>[2x]MAQVINTNSLSLITQNNINKNQSALSSSIERLSSGLRINSAKDDAAGQAIANRFTSNIKGLTQAARNANDGISVAQTTEGALSEINNNLQRIRELTVQASTGTNSDSDLDSIQDEIKSRLDEIDRVSGQTQFNGVNVLAKDGSMKIQVGANDGQTITIDLKKIDSDTLGLNGFNVNGKGETANTAATLKDMSGFTAAAAPGGTVGVTQYTDKSAVASSVDILNAVAGADGNKVTTSADVGFGTPAAAVTYTYNKDTNSYSAASDDISSANLAAFLNPQARDTTKAT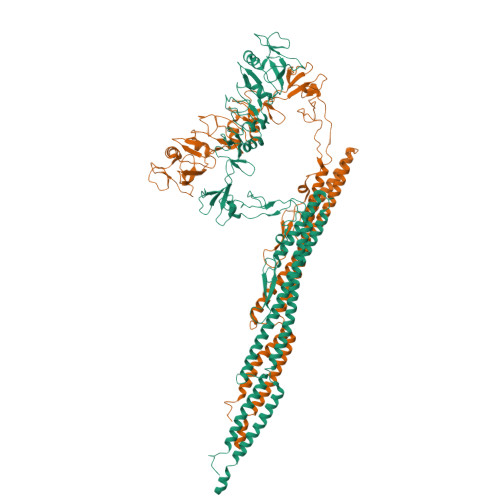VTIGGKDQDVNIDKSGNLTAADDGAVLYMDATGNLTKNNAGGDTQATLAKVATATGAKAATIQTDKGTFTSDGTAFDGASMSIDANTFANAVKNDTYTATVGAKTYSVTTGSAAADTAYMSNGVLSDTPPTYYAQADGSITTTEDAAAGKLVYKGSDGKLTTDTTSKAESTSDPLAALDDAISQIDKFRSSLGAVQNRLDSAVTNLNNTTTNLSEAQSRIQDADYATEVSNMSKAQIIQQAGNSVLAKANQVPQQVLSLLQG> MAE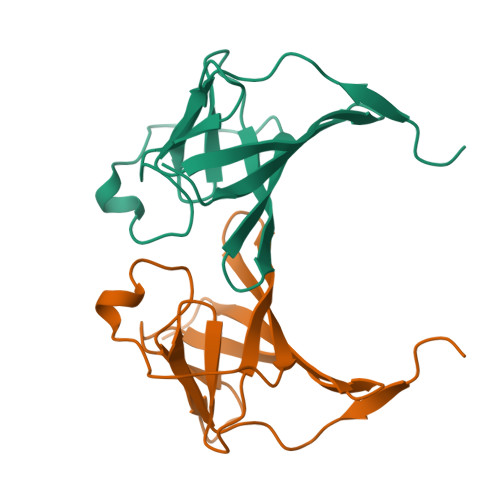CPTLGEAVTDHPDRLWAWEKFVYLDEKQHAWLPLTIEIKDRLQLRVLLRREDVVLGRPMTPTQIGPSLLPIMWQLYPDGRYRSSDSSFWRLVYHIKIDGVEDMLLELLPDD> DQCASSPCQNGGSCKD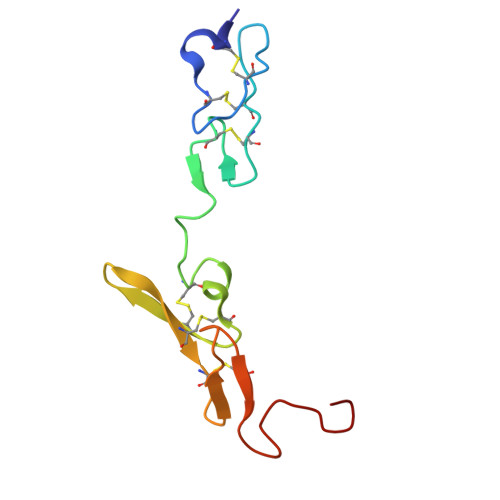QLQSYICFCLPAFEGRNCETHKDDQLICVNENGGCEQYCSDHTGTKRSCRCHEGYSLLADGVSCTPTVEYPCGKIPILE> FQGSESQLSVRVTPANAALKANIEAYVGSLGERDEAALQRFRRNAEAQAEKAAQALGYFQAQIDSEVKDGKPPKLTLKVVPGEPVRLRQVNIQVLGEAASLESFRLPSGKQLKPGAKLNQGVYEDAKRLIQNQASRYGFFQGRFSTQRLSIDPRAGIADIDLVYDSGQRYTFGKVSFDGDSIIEEELLRRMVPFKAGQPYDSELIAELNQNLQSSGYFEGVRVDAAPTQAQADGARQAIPVAVRLEARKPRTMGVGLGFSTDVGARA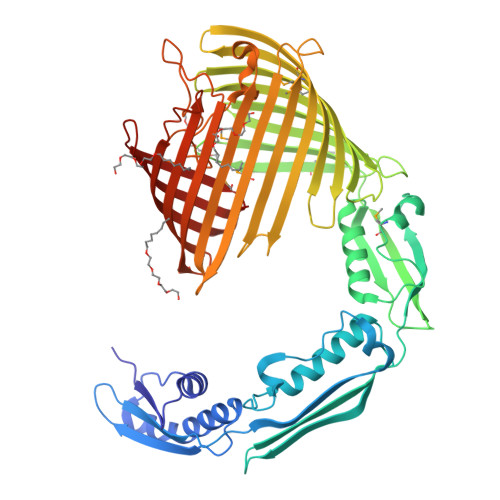RFNWTRHWVNAEGHSLGFESEISAPRQNVGAWYEIPLDPPLTDKLRFTSGYQFEDLVDTESKLLTLGGEWHSKRPDGWQRVVSLNWMREEYKLGDDSGLSSFLMPGIGYSLLETDNKVDPSHGYRLQFNVKGAKEGLLADADVLHVDAMAKGLTSFAGGHRLLGRLQVGGIATNDYKSIPPSLRFFAGGDQSVRGYDYRTLSPENSDGDKIGGRYMIAGSVEYQYPLAERWRLATFVDQGNAFNSLDFPSIKTGVGFGVRWVSPVGPLRLDLAHALDDDGGFRLHFSMGPEL> HEGVFQRGAAMRKRTVYGQVDEKSSPTSTSTDLTMKTTTTYSQNLKEPPPSNVFIPKRRIVHLDLKGAAPKPQHFRAFFEYFVRIGATGILIEWEDMFPYEGRLSDLRNGDAYSADDVRMILSTADQLRLEVIPLVQTIGHLEWLLKTHKFYSFRENPRNPQSVCVSNAEAVDLVLHLVDQVMAFHKDYGQFVHIGADEVYQYGECSRCVARMNKENLRREDLLLRHIVNVSKHVKTKYGKNVLMWHDMIANIDASLAEKYDLKNLVEPVLWNYAEDLEAFLPMGIWETFSAMVPYMWGSSAFKGADSPTRYHSNVKHYLENHISWIKQMSTASEKFREFRGLIFTGWQRYDHFAVLCEFLPIGIPSLTVNMLTIRNGRFDASVNDQAISIMQCVTGSDVKGDLYGCRFPGSDIYHHVQLLHEKKGEIEKLLLQQSVQGWLSNIAIDYNMSSPWYMNLIVPDLMTYKNQMIELSLNIRQAMLEMFYENAVDEFLFTYVDPVINHLQRLLDRATAIQRRDEFPVRPFPIKRTIDTTRAVDHHHHHH

Hexosaminidases are enzymes ubiquitous across all domains of life and play multiple roles in glycoconjugate metabolism as they remove nonreducing terminal N-acetylgalactosamine and N-acetylglucosamine residues from glycans, glycolipids, glycoproteins, and glycosaminoglycans. We have expressed one of these, HEX-2 from Trichuris suis, a porcine parasite, and shown that it prefers an aryl β-N-acetylgalactosaminide in vitro. Toward N-glycan substrates, it displays a preference for the removal of GalNAc residues from LacdiNAc motifs as well as the GlcNAc attached to the α1,3-linked core mannose. Therefore, a thorough phylogenetic analysis was performed and the GH20 subfamily 1 candidate enzyme from T. suis was expressed recombinantly, characterized, and successfully crystallized, yielding the first experimental structure of a eukaryotic subfamily 1 GH20 hexosaminidase.

In order to gain insight into the specificity of T. suis HEX-2, we solved its X-ray crystal structure at a resolution of 2.55 Å in a C2 space group. Overall, HEX-2 displays a modular structure with a N-terminal catalytic domain taking the shape of an (β/α)8 or TIM barrel followed by a C-terminal three helix bundle, whose function remains unknown. There is one protomer in the asymmetric unit. Analysis of the interfaces and assemblies with PDBePISA37 revealed one interface leading to the formation of a crystallographic dimer around the 2-fold axis. The structure also revealed the presence of a Zn2+ ion not far from the binding pocket. There is also a disordered surface loop between the Zn2+ site and the binding site which resulted in the lack of electron density between residues Glu199 and Arg220 so they could not be modeled. Additionally, the positioning of the Zn2+ ion implies a noncatalytic/structural role, potentially in the stabilization of this disordered loop upon substrate binding. As the enzymatic activity experiments indicated that T. suis HEX-2 removes GalNAc and GlcNAc residues from glycan substrates, its newly resolved catalytic domain was superimposed on that of S. pneumoniae GH20C, which has been cocrystallized with the GalNAc and GlcNAc reaction products, which are also surrogates for actual substrates. 265 residues out of 320 aligned with a rmsd of 1.9 Å and major differences are observed at the level of surface loops in particular those surrounding the active site pocket and in particular the −1 subsite. This structural analysis indicated that either monosaccharide is capable of effectively binding to the predicted −1 subsite, whereby the key contacts will be conserved with the 1-hydroxyl and 2-acetamido groups.>[2x]FFFDGSTLEGYYVDDALQGQGVYTYEDGGVLQGTYVDGELNGPAQEYDTDGRLIFKGQYKDNIRHGVCWIYYPDGGSLVGEVNEDGEMTGEKIAYVYPDERTALYGKFIDGEMIEGKLATLMSTEEGRPHFELMPGNSVYHFDKSTSSCISTNALLPDPYESERVYVAESLISSAGEGLFS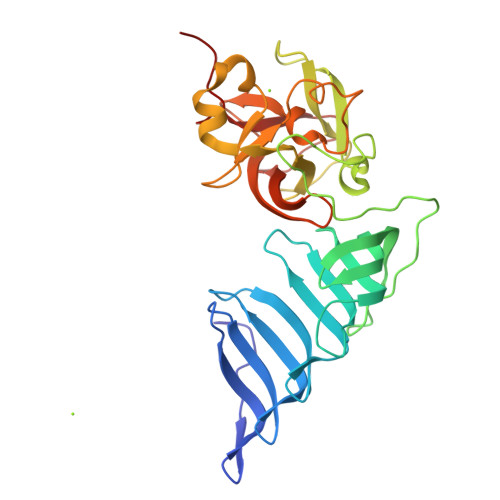KVAVGPNTVMSFYNGVRITHQEVDSRDWALNGNTLSLDEETVIDVPEPYNHVSKYCASLGHKANHSFTPNCIYDMFVHPRFGPIKCIRTLRAVEADEELTVAYGYDHSPPGK> MTIDDSNRLLMDVDQFDFLDDGTAQLSNNKTDEEEQLYKRDPVSGAILVPMTVNDQPIEKNGDKMPLKFKLGPLSYQNMAFITAKDKYKLYPVRIPRLDTSKEFSAYVSGLFEIYRDLGDDRVFNVPTIGVVNSNFAKEHNATVNLAMEAILNELEVFIGRVKDQDGRVNRFYELEESLTVLNCLRTMYFILDGQDVEENRSEFIESLLNWINRSDGEPDEEYIEQVFSVKDSTAGKKVFETQYFWKLLNQLVLRGLLSQAIGCIERSDLLPYLSDTCAVSFDAVSDSIELLKQYPKDSSSTFREWKNLVLKLSQAFGSSATDISGELRDYIEDFLLVIGGNQRKILQYSRTWYESFCGFLLYYIPSLELSAEYLQMSLEANVVDITNDWEQPCVDIISGKIHSILPVMESLDSCTAAFTAMICEAKGLIENIFEGEKNSDDYSNEDNEMLEDLFSYRNGMASYMLNSFAFELCSLGDKELWPVAIGLIALSATGTR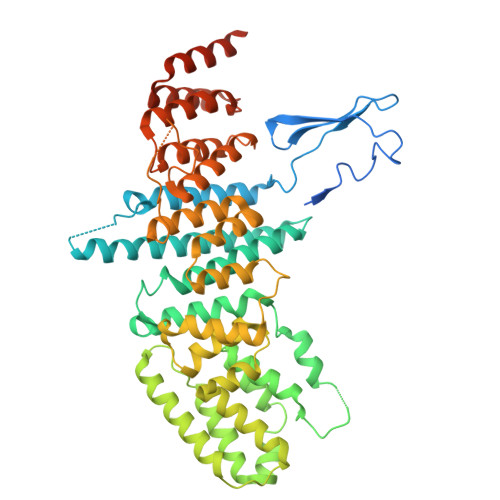SAKKMVIAELLPHYPFVTNDDIEWMLSICVEWRLPEIAKEIYTTLGNQMLSAHNIIESIANFSRAGKYELVKS4-[2-(4-propan-2-ylphenyl)ethyl]-1-[(~{E})-prop-1-enyl]piperidine 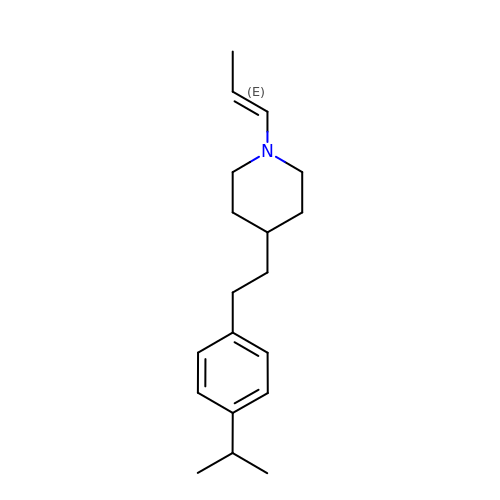| C19 H29 N | ZAGXDKMVGYZZKY-YIXHJXPBSA-N> AYL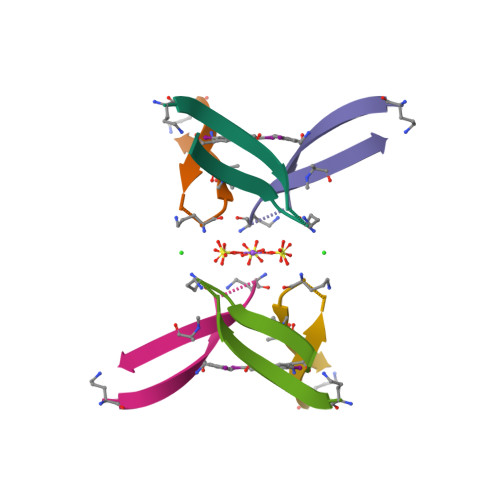LFYVEAKVAAAVK> MAAYTDVPISGMRKTIAARLKESVTENPHFFVSTNLSVSKLLKLRQALNSSADGRYKLSVNDFLIKAMGIASKRVPTVNSSWRDGVIRQFETVDVSVAVATPNGLITPIVKGVEGKGLESISAAVKELAKKARDGKLKPEEYQGGSISISNMGMNPAVQSFTAIINPPQAAILAVGAPQKVAVPVENEDGTTGVSWD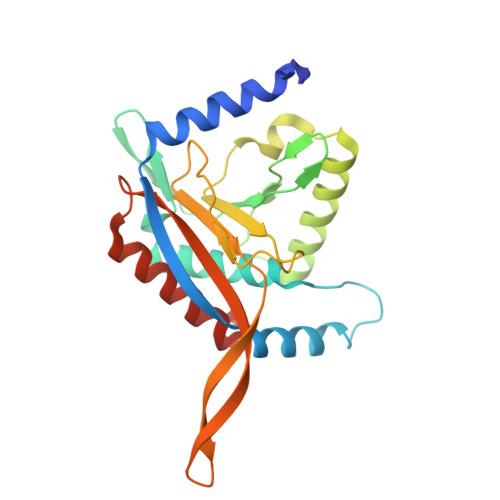EQIIVTASFDHKVVDGAVGAEWIRELKKVIENPLELLL(2~{R},3~{R},4~{S},5~{R})-2-(6-aminopurin-9-yl)-5-[[3-[6-azanyl-9-[(2~{R},3~{R},4~{S},5~{R})-5-(hydroxymethyl)-3,4-bis(oxidanyl)oxolan-2-yl]purin-8-yl]prop-2-ynyl-methyl-amino]methyl]oxolane-3,4-diol 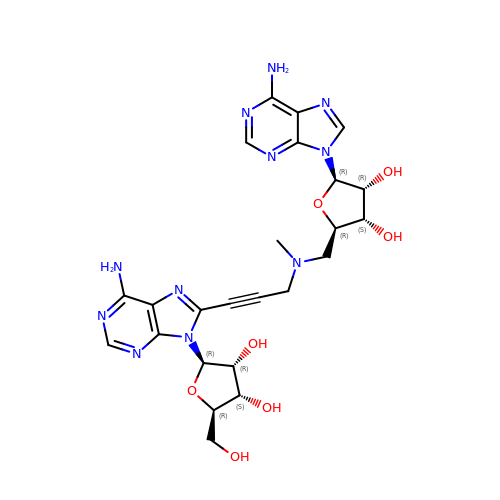| C24 H29 N11 O7 | OPWBYPZWGGCZGG-KRSQEUQLSA-N>[3x]ASAKELACQEITVPLCKGIGYNYTYMPNQFNHDTQDEAGLEVHQFWPLVEIQCSPDLKF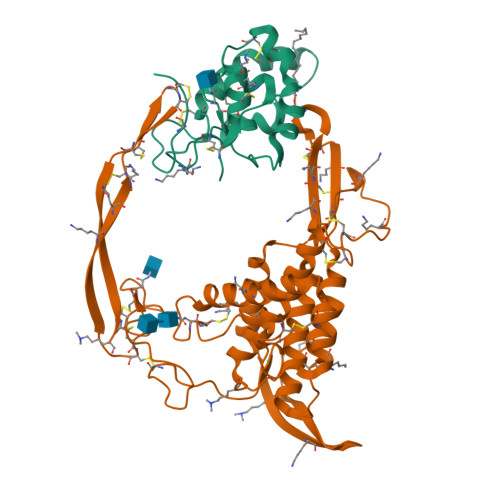FLCSMYTPICLEDYKKPLPPCRSVCERAKAGCAPLMRQYGFAWPDRMRCDRLPEQGNPDTLCMDYNRTDLTTASRPAPELLG;>GKDGSPLLCGSIPGLVPKQLRFCRNYIEIMPSVAEGVKLGIQECQHQFRGRRWNCTTIDDSLAIFGPVLDKATRESAFVHAIASAGVAFAVTRSCAEGTSTICGCDSHHKGPPGEGWKWGGCSEDADFGVLVSREFADARENRPDARSAMNKHNNEAGRTTILDHMHLKCKCHGLSGSCEVKTCWWAQPDFRAIGDFLKDKYDSASEMVVEKHRESRGWVETLRAKYSLFKPPTERDLVYYENSPNFCEPNPETGSFGTRDRTCNVTSHGIDGCDLLCCGRGHNTRTEKRKEKCHCIFHWCCYVSCQECIRIYDVHTCK[3x]>PALTKSQTDRLEVLLNPKDEISLNSGKPFRELESELLSRRKKDLQQIYAEERENYLGKLEREITRFFVDRGFLEIKSPILIPLEYIERMGIDNDTELSKQIFRVDKNFCLRPMLAPNLYNYLRKLDRALPDPIKIFEIGPCYRKESDGKEHLEEFTMLDFSQMGSGCTRENLESIITDFLNHLGIDFKIVGDSCMVFGDTLDVMHGDLELSSAVVGPIPLDREWGIDKPWIGAGFGLERLLKVKHDFKNIKRAARSES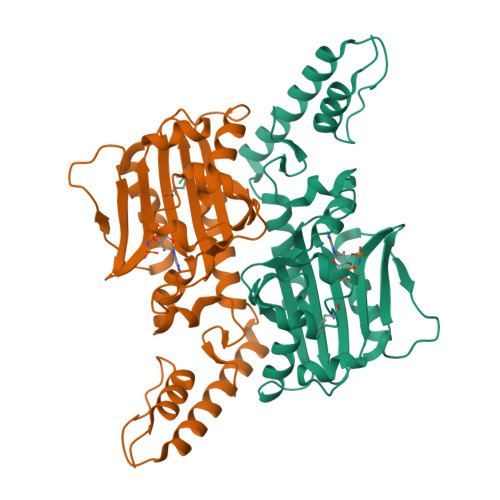YYNGISTNL[4x]SulE, an esterase, which detoxifies a variety of sulfonylurea herbicides through de-esterification, provides an attractive approach to remove environmental sulfonylurea herbicides and develop herbicide-tolerant crops. SulE catalyzes the de-esterification of a variety of sulfonylurea herbicides, such as MM, BM, SM, TM, TrM, EM, and CE, to the corresponding herbicidal-inactive parent acid. The structures show that SulE is a dimer with a lid loop in a domain-swapped β-hairpin covering the active site from the opposing monomer. SulE shows a similar catalytic triad consisting of Ser209, His333, and Glu232 at its active site.

To understand the molecular basis for the altered activity by Pro44 mutation, the crystal structures of apo-P44R, the double mutant P44R/S209A in complex with CA, and the triple mutant P44R/S209A/H333A in complex with MM, CE, and TM were determined in the range of 1.32–1.78 Å. In the structure of P44R/S209A in complex with CA, each subunit bound a CA molecule in the substrate binding pocket; unexpectedly, an extra CE molecule bound to the interface of the dimer and also interacted with the symmetric molecule B. This CE molecule does not cause any change in protein conformation, suggesting that it may only play a role in crystal packing. A clear electron density was also observed for the full CA molecule in the active site of P44R/S209A. Structural comparison showed that CA and CE are well superimposed, indicating that binding the product also induces the conformational change in the structures containing the P44R mutation. However, it was found that the SulE S209A and P44R/S209A mutants still retained weak activity in this study. The distance between His333 and the substrate is too long to have a direct reaction; therefore, the reason why SulE S209A and P44R/S209A mutants still retain de-esterification activity may be that a water molecule got into the active site and was directly deprotonated by His333 when Ser209 is mutated to alanine, and then as a nucleophile to attack the ester bond of the substrate. Supporting this, a water molecule was found in the active site of the P44R/S209A-CA complex structure, which may serve as a nucleophile.

>[2x]METDNVELAQSKRKVVLAEQGSFYIGGRTVTGPGKFDPSKPVIRYSNEGATFYINQMYVNFQAPVRPRGLPLVFWHGGGLTGHIWESTPDGRPGFQTLFVQDRHTVYTIDQPGRGRGNIPTFNGPFGQLEEESIVNTVTGNSSKEGAWVRDRLGPAPGQFFENSQFPRGYEDNYFKEMGFSPSISSDEIVDAVVKLVTHIGPCVLVTHAASGVLGMRVATHAKNVRGIVAYEPATSIFPKGKVPEIPPLADKKSQIFPPFEIQESYFKKLAKIPIQFVFGDNIPKNPKSAYWFLDWWRVTRYAHSLSLEAINKLGGQASLLDLPTAGLRGNTHFPFTDRNNVQVASLLSDFLGKHGLDQNESLEHHHHHH> MKKKPFSILFMGIEDYATKGQKGRSDSLIVVTLDPKNKTMKMLSIPRDTRVQLAGDTTGSKTKINAAYSKGGKDETVETVENFLQIPIDKYVTVDFDGFKDVINEVGGIDVDVPFDFDEKSDVDESKRIYFKKGEMHLNGEEALAYARMRKQDKRGDFGRNDRQKQILNALIDRMSSASNIAKIDKIAEK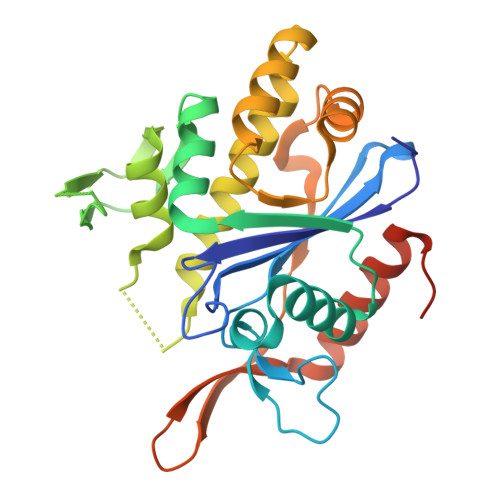ASENVETNIRITEGLALQQIYSGFTSKKIDTLSITGSDLYLGPNNTYYFEPDATNLEKVRKTLQEHLDYTPLEHHHHHHHH>[6x]MRATKHILILILLVFLVISCKNKQSNTQNPNQQNQNEVTAKDILGNSKYLAISYGGYRKKSRDFQPSI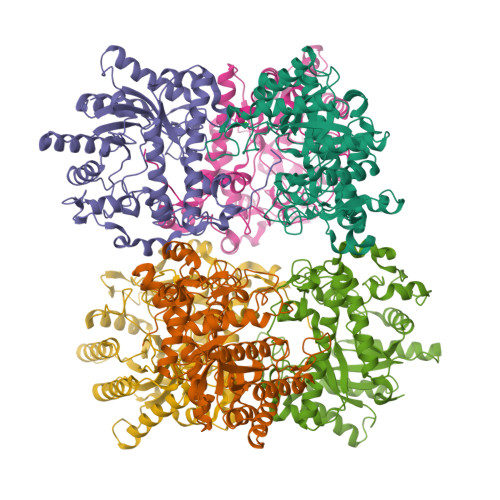EELKEDMKILHAMNIRILRTYNVRLAHTSNILKAIRELKNEDANFEMYMMVGAWIDCKNAWTDQPLNHHEESENNASEIDRAVALAQEFPDIVKVIAVGNEAMVKWAASYFVQPAVILKWVNHLQALKKKGDLSKDLWITSSDNFASWGGGDPQYHVEDLTKLIEAVDYLSVHTYPMHDTHYNPIFWGVFGDETELSSLKRIDIAMNRAKTYAVSQSDSVASYIKSLGINKPIHIGETGWASFSNGYYGAKGSKATDEYKEAIFYNHIREWTNEANMSCFYFEAFDEPWKDAHNSGGSENHFGLFTVDGKAKYVLWDLVDKGVFEGLTRGGNPITKTYNGNKEALFLEVELPPVKKEITKNH> GGSEVRILLLGLDNAGKTTLLKQLASEDISHITPTQGFNIKSVQSQGFKLN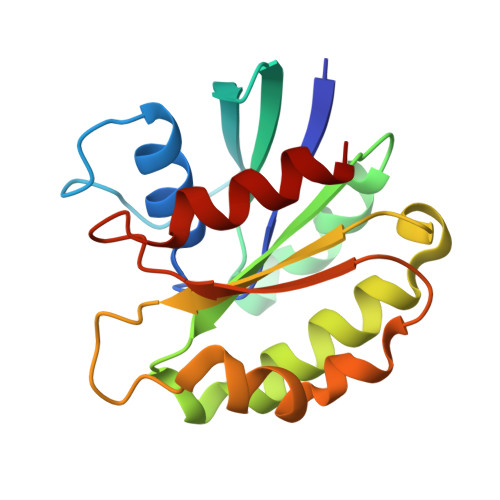VWDIGGLRKIRPYWRSYFENTDILIYVIDSADRKRFEETGQELTELLEEEKLSCVPVLIFANKQDLLTAAPASEIAEGLNLHTIRDRVWQIQSCSALTGEGVQDGMNWVCKNV[(2~{R},3~{R},4~{R},5~{R})-5-(2-azanyl-7-methyl-6-oxidanylidene-1~{H}-purin-7-ium-9-yl)-4-methoxy-3-oxidanyl-oxolan-2-yl]methyl 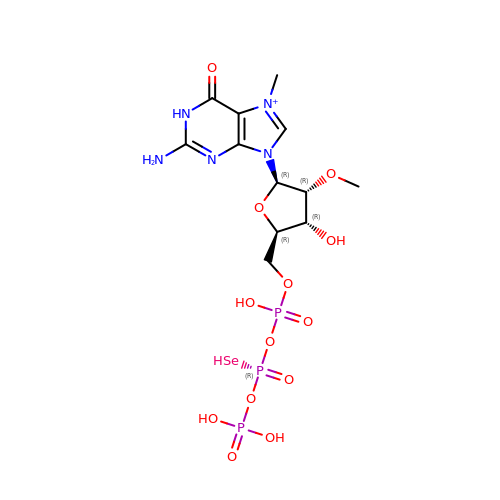[phosphonooxy(selanyl)phosphoryl] hydrogen phosphate | C12 H21 N5 O13 P3 Se | FCPLZYTYUZTIIR-ZRDSBRMSSA-O>[7x]MAGLYTTYQLLEVQRKLKTLPAFFLQWFPRQINFQEDMIAFDKVIQDVTRVAPF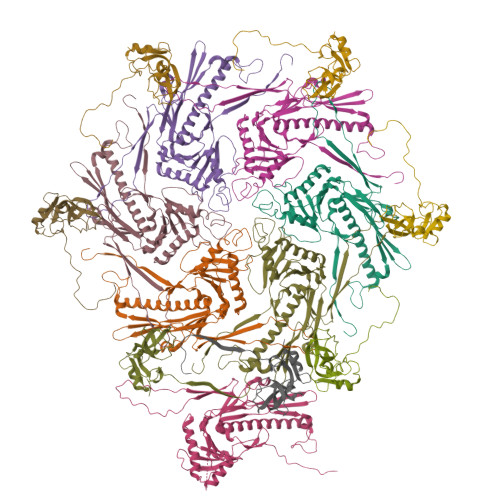VAPNVQGRVIKESGYNTKTFKPAYVKPKHVIDPNMIIPRQPGEALGTGTLSIAQRRDRVIAYLLMKHRAMHENTWEWMAAQAAQYGYVDVQGQDYPLVRVDFGRDAALTMTTDWTAAGVTLMDMIADLRDGQRLVSDKSMSGTVIRDYIFGGDAWDQFVKVGGKELWGKDGLMDSTIRGSETNVTRLWDDVEGVQYMGELVGANGAGRMRIWVNTQKYRDQNDQEQFLMKQKAVMGISSAIEGVRCFGAILDKGAGYQALDYFPKMWDQEDPSVEYLMSQGAPLMVPADPNASFLLTVMS;>[7x]MNLLTMMAATSLPNYLAGNGDLGSWEPTQIFAGEADIVTEGGAAGADIEIYQVIAKNAAGAMVPHDPTATTGTSPDEVPAPQSVAIGIAAQPAKSGQNVPYYIGGVFNHAALGWHASLDTLAKRQAVFDRTNIHIGNLY>DVNTNIVLGGTTAPAVKGDVNVTSNVQAITSPQTTTIDNQTGAVTYSNWDGKVNGTVTATYNGQSYTATLNETAGKENSRVTPWYTQDGGKTWNVLKKDGGVYRLEPAGKYQLSVNNVSFNFGTANANKKNITLTSSNGVQFRENGQWKDSIK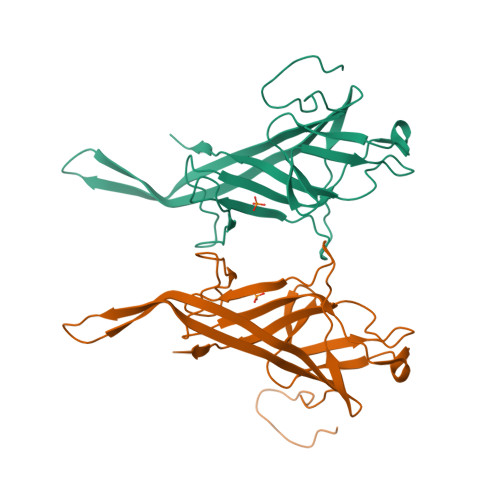VSTDQNGAVSQPLTLLIPITPVDVTNAKS[2x]>[2x]TEEKTCDLVGEKGKESEKELALLKRLTPLFQKSFESTVGQSPDMYSYVFRVCREAGQHSSGAGLVQIQKSNGKETVVGR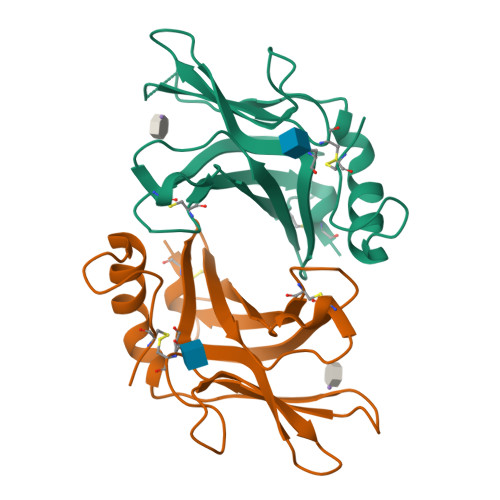FNETQIFQGSNWIMLIYKGGDEYDNHCGREQRRAVVMISCNRHTLADNFNPVSEERGKVQDCFYLFEMDSSLACS> CELDRDPEGKDFQQPYTSFVQTKQNRDGLYALLRNTENPRMHFYQELQSDMYCTTITDGNSLAPFVNWDLGILNDHGRADEDEVSGIAGYYFVYNRLNQQANAFVNNTEAALQNQVYKNSTEIANAKSFLAEGKVLQALAIWRLMDRFSFHESVTEVNSGAKDLGVILLKEYNPGYIGPRATKAQCYDYILSRLSEAIEVLPENRESVLYVSRDYAYALRARIYLALGEYGKAAADAKMVVDKYPLIGAADASEFENIYRSDANNPEIIFRGFASATLGSFTATT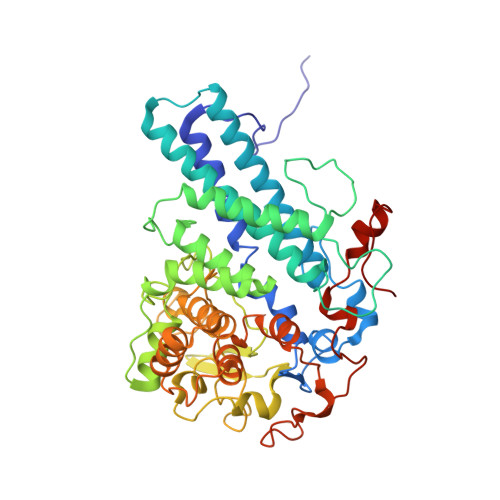LNGAAPAGKDIKYNPSAVPFQWVVDLYENEDFRKSVYIAKVVKKDKGYLVNKFLEDKAYRDVQDKPNLKVGARYFSVAEVYLILVESALQTGDTPTAEKYLKALSKARGAEVSVVNMEALQAERTRELIGEGSRLRDMVRWSIPNNHDAFETQPGLEGFANTTPLKAQAPVGFYAYTWEFPQRDRQTNPQLIKNWPIHHHHHH COENZYME A PERSULFIDE | C21 H36 N7 O16 P3 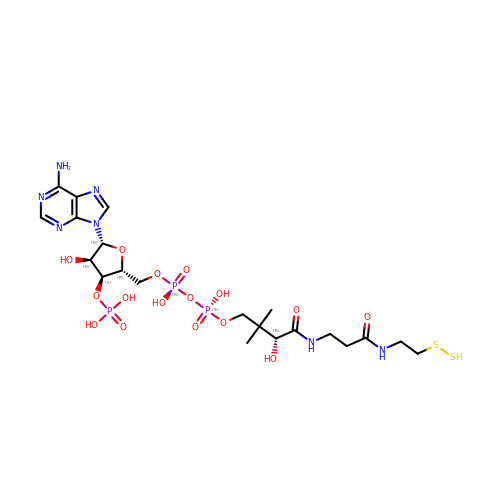S2 | REVPHPVBPSIEKM-IBOSZNHHSA-N>[2x]MSR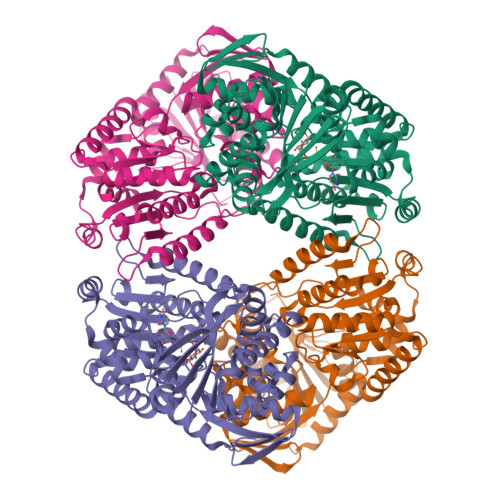LVVVSNRIAPPDEHAASAGGLAVGILGALKAAGGLWFGWSGETGNEDQPLKKVKKGNITWASFNLSEQDLDEYYNQFSNAVLWPAFHYRLDLVQFQRPAWDGYLRVNALLADKLLPLLQDDDIIWIHDYHLLPFAHELRKRGVNNRIGFFLHIPFPTPEIFNALPTYDTLLEQLCDYDLLGFQTENDRLAFLDCLSNLTRVTTRSAKSHTAWGKAFRTEVYPIGIEPKEIAKQAAGPLPPKLAQLKAELKNVQNIFSVERLDYSKGLPERFLAYEALLEKYPQHHGKIRYTQIAPTSRGDVQAYQDIRHQLENEAGRINGKYGQLGWTPLYYLNQHFDRKLLMKIFRYSDVGLVTPLRDGMNLVAKEYVAAQDPANPGVLVLSQFAGAANELTSALIVNPYDRDEVAAALDRALTMSLAERISRHAEMLDVIVKNDINHWQECFISDLKQIVPRSAESQQRDKVATFPKLALEHHHHHH5-methylnaphthalene-1-carboxylic acid | C12 H10 O2 | 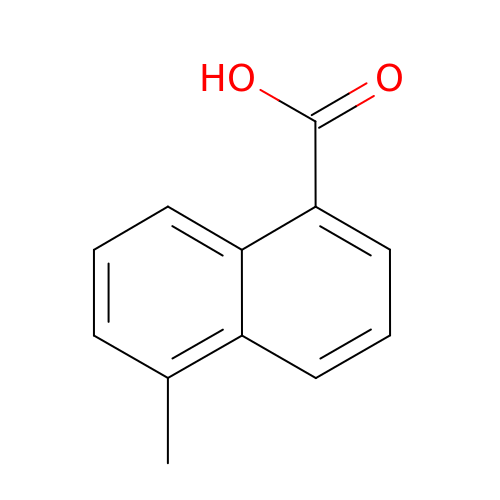VLEZTIKHFUAVRK-UHFFFAOYSA-N>MSQFFIRRPVFAWVIAIFIIIFGLLSIPKLPIARFPSVAPPQVNISATYPGATAKTINDSVVTLIERELSGVKNLLYYSATTDTSGTAEITATFKPGTDVEMAQVDVQNKIKAVEARLPQVVRQQGLQVEASSSGFLMLVGINSPNNQYSEVDLSDYLVRNVVEELKRVEGVGKVQSFGAEKAMRIWVDPNKLVSYGLSISDVNNAIRENNVEIAPGRLGDLPAEKGQLITIPLSAQGQLSSLEQFKNISLKSKTNGSVIKLSDVANVEIGSQAYNFAILENGKPATAAAIQLSPGANAVKTAEGVRAKIEELKLNLPEGMEFSIPYDTAPFVKISIEKVIHTLLEAMVLVFIVMYLFLHNVRYTLIPAIVAPIALLGTFTVMLLAGFSINVLTMFGMVLAIGIIVDDAIVVVENVERIMATEGLSPKDATSKAMKEITSPIIGITLVLAAVFLPMAFASGSVGVIYKQFTLTMSVSILFSALLALILTPALCATILKPIDGHHQKKGFFAWFDRSFDKVTKKYELMLLKIIKHTVPMMVIFLVITGITFAGMKYWPTAFMPEEDQGWFMTSFQLPSDATAERTRNVVNQFENNLKDNPDVKSNTAILGWGFSGAGQNVAVAFTTLKDFKERTSSASKMTSDVNSSMANSTEGETMAVLPPAIDELGTFSGFSLRLQDRANLGMPALLAAQDELMAMAAKNKKFYMVWNEGLPQGDNISLKIDREKLSALGVKFSDVSDIISTSMGSMYINDFPNQGRMQQVIVQVEAKSRMQLKDILNLKVMGSSGQLVSLSEVVTPQWNKAPQQYNRYNGRPSLSIAGIPNFDTSSGEAMREMEQLIAKLPKGIGYEWTGISLQEKQSESQMAFLLGLSMLVVFLVLAALYESWAIPLSVMLVVPLGIFGAIIAIMSRGLMNDVFFKIGLITIIGLSAKNAILIVEFAKMLKEEGMSLIEATVAAAKLRLRPILMTSLAFTCGVIPLVIATGASSETQHALGTGVFGGMISATILAIFFVPVFFIFILGAVEKLFSSKKKISS[3x]

In A. baumannii, the best-characterized multidrug efflux system is the prevalent Acinetobacter drug efflux ABC (AdeABC) tripartite system. This efflux system is capable of mediating resistance to a broad spectrum of clinically relevant antimicrobial agents, such as aminoglycosides, tetracyclines, macrolides, β-lactams, fluoroquinolones, chloramphenicol, and trimethoprim. The AdeABC locus consists of three tandemly linked genes encoding the AdeA periplasmic membrane fusion protein, the AdeB multidrug efflux pump, which is an inner membrane protein belonging to the hydrophobe-amphiphile efflux resistance-nodulation-cell division (HAE-RND) family of efflux transporters, and the AdeC outer membrane channel protein. Each subunit of AdeB contains 12 transmembrane helices (TM1 to TM12) and six periplasmic subdomains (PN1, PN2, PC1, PC2, DN, and DC).

Three distinct conformations of apo-AdeB (AdeB-I, AdeB-II, and AdeB-III) were captured in our cryo-EM data. Like AdeB-I, the three AdeB protomers of the second apo-AdeB structure, designated AdeB-II, present an extrusion conformation, where the three periplasmic clefts of the AdeB trimer are closed and a channel for extrusion is found in each protomer. However, in the AdeB-II structure, it is observed that the organization of the AdeB trimer is packed in a way that can be interpreted as a dimer plus monomer configuration within the transmembrane domain. The region that maintains the assembly of the pump in the trimeric oligomerization state is the periplasmic domain, where the long-arm feature formed by subdomain DN strongly coordinates with the hook-like structural feature of subdomain DC of the neighboring AdeB subunit to secure intersubunit interactions within the trimer. This region also contributes to form a hinge so that the transmembrane domain of each protomer is capable of shifting toward and away from each other. Within the two protomers interacting with each other at the transmembrane region, we observed three bound PE lipids. One of these lipids is located at the interface between the two AdeB protomers. The other two lipid molecules are found to bind by individual protomers. No lipid is observed to associate with the third AdeB protomer. We suspect that the switch in configuration of the trimeric AdeB pump from trimer to dimer plus monomer and monomer plus monomer plus monomer can alter the interactions between the AdeB pump and AdeA adaptor at the protein-protein interface, in turn facilitating the transport of substrates across the periplasmic space of A. baumannii.>[2x]MFDFDGYMLRKAKSVNKALEAAVQMKEPLKIHESMRYSLLAGGKRVRPMLCIAACELVGGDESTAMPAACAVEMIHTMSLMHDDLPCMDNDDLRRGKPTNHMAFGESVAVLAGDALLSFAFEHVAAATKGAPPERIVRVLGELAVSIGSEGLVAGQVVDVCSEGMAEVGLDHLE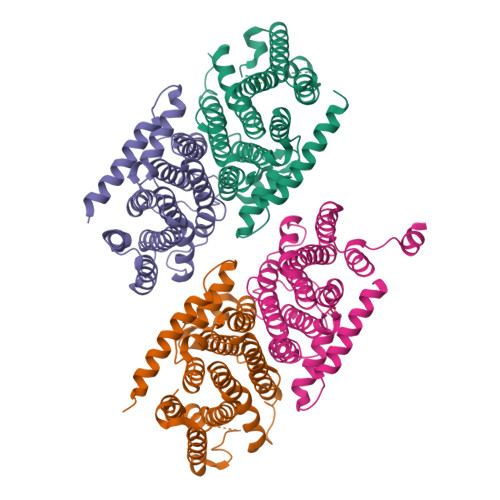FIHHHKTAALLQGSVVLGAILGGGKEEEVAKLRKFANCIGLLFQVVDDILDVTKSSKELGKTAGKDLVADKTTYPKLIGVEKSKEFADRLNREAQEQLLHFHPHRAAPLIALANYIAYRDN;>MQPYWAAIEADIERYLKKSITIRPPETVFGPMHHLTFAAPATAASTLCLAACELVGGDRSQAMAAAAAIHLVHAAAYVHEHLPLTDGSRPVSKPAIQHKYGPNVELLTGDGIVPFGFELLAGSVDPARTDDPDRILRVIIEISRAGGPEGMISGLHREEEIVDGNTSLDFIEYVCKKKYGEMHACGAACGAILGGAAEEEIQKLRNFGLYQGTLRGMMEMKNSHQLIDENIIGKLKELALEELGGFHGKNAELMSSLVAEPSLYAAHHHHHHHH[2x]1-[(2R)-2-[(2,4-dichlorobenzyl)oxy]-2-(2,4-dichlorophenyl)ethyl]-1H-imidazole 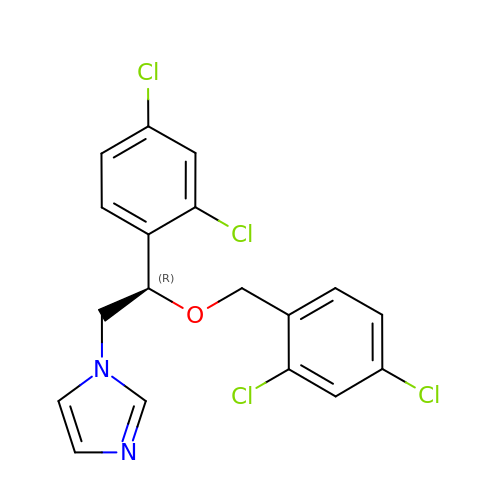| C18 H14 Cl4 N2 O | BYBLEWFAAKGYCD-SFHVURJKSA-N>HMQSRELKTVSADCKKEAIEKCAQWVVRDCRPFSAVSGSGFIDMIKFFIKVGAEYGEHVNVEELLPSPITLSRKVTSDAKEKKALIGREIKSAVEKDGASATIDLWTDNYIKRNFLGVTLHYHENNELRDLILGLKSLDFERSTAENIYKKLKAIFSQFNVEDLSSIKFVTDRGANVVKSLANNIRINCSSHLLSNVLENSFEETPELNMPILACKNIVKYFKKANLQHRLRSSLKSECPTRWNSTYTMLRSILDNWESVIQILSEAGETQRIVHINKSIIQTMVNILDGFERIFKELQTCSSPSLCFVVPSILKVKEICSPDVGDVADIAKLKVNIIKNVRIIWEENLSIWHYTAFFFYPPALHMQQEKVAQIKEFCLSKMEDLELINRMSSFNELSATQLNQSDSNSHNSIDLTSHSKDISTTSFFFPQLTQNNSREPPVCPSDEFEFYRKEIVILSEDFKVMEWWNLNS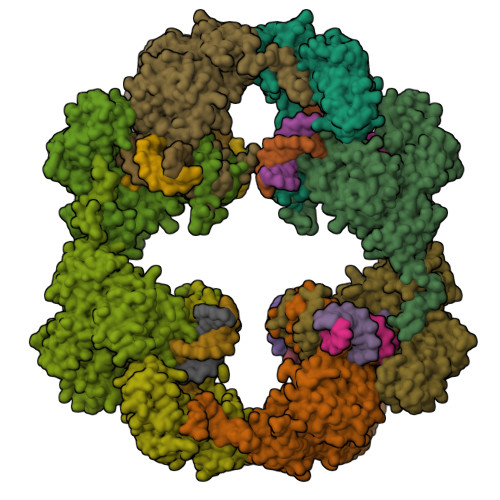KKYPKLSKLALSLLSIPASSAASERTFSLAGNIITEKRNRIGQQTVDSLLFLNSFYKNFCKLDI[4x]>HMASMTGGQQMGRGSDFGDIEERGKILVSLMYSTQQGGLIVGIIRCVHLAAMDANGYSDPFVKLWLKPDMGKKAKHKTQIKKKTLNPEFNEEFFYDIKHSDLAKKSLDISVWDYDIGKSNDYIGGCQLGISAKGERLKHWYECLKNKDKKIERWHQLQNENH[6x];>GSHMASMTGGQQMGRGSEFMRNELEEMQRRADQLADESLESTRRMLQLVEESKDAGIRTLVMLDEQGEQLDRVEEGMNHINQDMKEAEKNLKDLG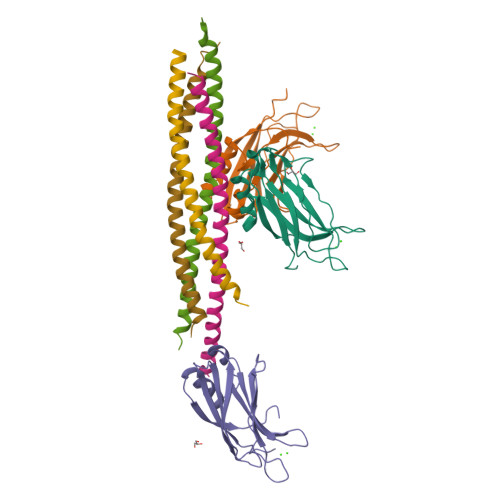[4x];>GSHMASMTGGQQMGRGSEFARENEMDENLEQVSGIIGNLRHMALDMGNEIDTQNRQIDRIMEKADSNKTRIDEANQRATKML[4x]>MGGSRSLSAFSPPLPCDPARSHPTPEFPSSLQDYCEIRGIQSQPPARRDPTMDWLASLRSQIKPYRDRFPSHARLPRAGLPRAEILAEIAAMGAA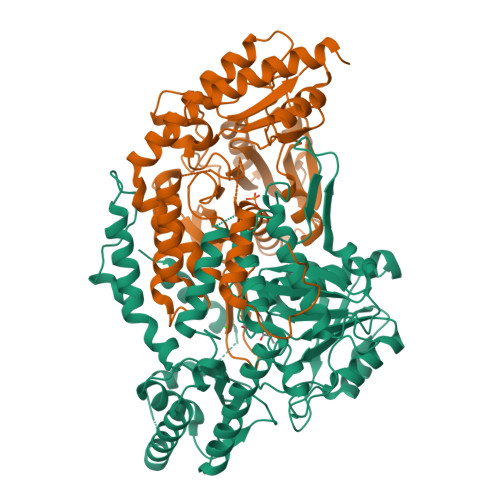ESPAWRDGYASGAVYHGDEHHIAFLNEVYALQSQSNPLHPDLWPSTAKFEAEVVAMTAHMLGGDAAGGTVCGTVTSGGTESLLLAMKTYRDWARATKGITAPEAVVPVSAHAAFDKAAQYFGIKLVRTPLDADYRADVAAMREAITPNTVVVAGSAPGYPHGVVDPIPEIAALAAEHGIGCHVDACLGGFILPWAERLGYPVPPFDFRLEGVTSVSADTHKYGYGAKGTSVILYRRPDLLHYQYFIAADWPGGLYFSPTFAGSRPGALSATAWAAMLSLGEEGYLDATRRILQAADRLKAGVRAIPSLKILGDPLWVIAVASDELNIYQVMEEMAGRGWRLNGLHRPPAFHVALTLRHTEPGVVDRFLADLQDAVAQVRAHPEKATGMAPVYGMAAAAPPELVRQVLTGFIDLLYEVHHHHHH[2x]> MKITVWTHFGGPELEWLKEQARTFERTSGTKVEVVEVPFAEIKQKFILGAPQGQAADLVVTVPHDWVGEMAQAGVLEPVGKYVTQAYLADLQGVAVEAFTFGGRLMGLPAFAESVALIYNKKYVKEPPRTWEEFLALA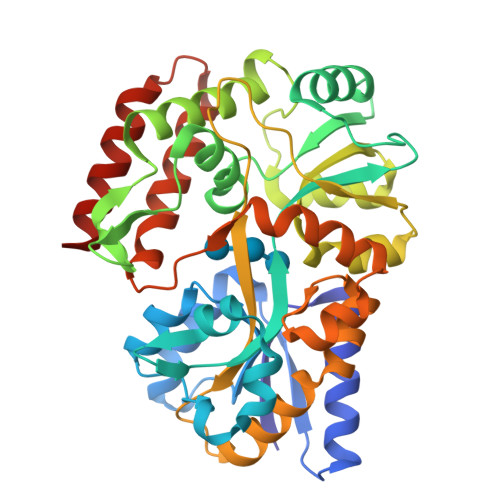QKLTTGATFGFLYNIGDPYFNFGFFKAFGAENVFAKDAKGNLDPTKLLIGGEVGEKALQFIKDLRFKYNLVPEGVDYGVADGAFKDGALAMILNGPWALGDYKKAKVDFGIAPFPVPPGAKNPWGPFLGVQGVVVNAYSKNKTQAVNFAKTLVTGRNLVAFNQAGGRIPVSKSAVKQLEKDPVVAGFSKVFPLGAPMPNIPEMGKVWGPWGNAISLAIQRPDSNVKKIVEDMVAEIKKAIGRHHHHHH>[3x]MIQGVIQKIAGPAVIAKGMLGARMYDICKVGEEGLVGEIIRLDGDTAFVQVYEDTSGLKVGEPVVSTGLPLAVELGPGMLNGIYDGIQRPLERIREKTGIYITRGVVVHALDREKKWAWTPMVKPGDEVRGGMVLGTVPEFGFTHKILVPPDVRGRVKEVKPAGEYTVEEPVVVLEDGTELKMYHTWPVRRARPVQRKLDPNTPFLTGMRILDVLFPVAMGGTAAIPGPFGSGKTVTQQSLAKWSNADVVVYVGCGERGNEMTDVLVEFPELTDPKTGGPLMHRTVLIANTSNMPVAAREASIYVGVTIAEYFRDQGFSVALMADSTSRWAEALREISSRLEEMPAEEGYPPYLAARLAAFYERAGKVITLGGEEGAVTIVGAVSPPGGDMSEPVTQSTLRIVGAFWRLDASLAFRRHFPAINWNGSYSLFTSALDPWYRENVAEDYPELRDAISELLQREAGLQEIVQLVGPDALQDAERLVIEVGRIIREDFLQQNAYHEVDAYCSMKKAYGIMKMILAFYKEAEAAIKRGVSIDEILQLPVLERIGRARYVSEEEFPAYFEEAMKEIQGAFKALA;>MDLLKKEYTGITYISGPLLFVENAKDLAYGAIVDIKDGTGRVRGGQVIEVSEEYAVIQVFEETTGLDLATTSVSLVEDVARLGVSKEMLGRRFNGIGKPIDGLPPITPEKRLPITGLPLNPVARRKPEQFIQTGISTIDVMNTLVRGQKLPIFSGSGLPANEIAAQIARQATVRPDLSGEGEKEEPFAVVFAAMGITQRELSYFIQEFERTGALSRSVLFLNKADDPTIERILTPRMALTVAEYLAFEHDYHVLVILTDMTNYCEALREIGAAREEIPGRRGYPGYMYTDLATIYERAGVVEGKKGSVTQIPILSMPDDDRTHPIPDLTGYITEGQIQLSRELHRKGIYPPIDPLPSLSRLMNNGVGKGKTREDHKQVSDQLYSAYANGVDIRKLVAIIGEDALTENDRRYLQFADAFERFFINQGQQNRSIEESLQIAWALLSMLPQGELKRISKDHIGKYYGQKLEEIWGAPQALD[3x];> MSQVSPTRMNLLQRRGQLRLAQKGVDLLKKKRDALVAEFFGLVREAMEARKALDQAAKEAYAALLLAQAFDGPEVVAGAALGVPPL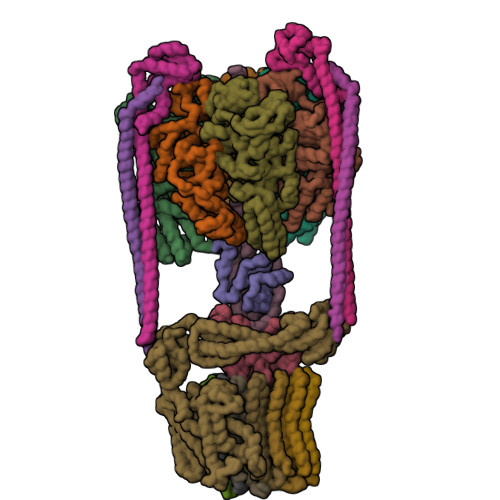EGVEAEVENVWGSKVPRLKATFPDGALLSPVGTPAYTLEASRAFRRYAEALIRVANTETRLKKIGEEIKKTTRRVNALEQVVIPGIRAQIRFIQQVLEQREREDTFRLKRIKGKIEAREAEEEGGRPNPQVEIGAGL;> MAVIADPETAQGFRLAGLEGYGASSAEEAQSLLETLVERGGYALVAVDEALLPDPERAVERLMRGRDLPVLLPIAGLKEAFQGHDVEGYMRELVRKTIGFDIKL;>MTGGLVLNAISRAGGAMGGLGLIKSLAEKEKQLLERLEAAKKEAEERVKRAEAEAKALLEEAEAKAKALEAQYRERERAETEALLARYRERAEAEAKAVREKAMARLDEAVALVLKEVLP[2x];>[2x]MSKLEAILSQEVEAEIQALLQEAEAKAEAVKREAEEKAKALLQARERALEAQYRAALRRAESAGELLVATARTQARGEVLEEVRRRVREALEALPQKPEWPEVVRKLALEALEALPGAKALVANPEDLPHLEAMARERGVELQAEPALRLGVRAVGAEGKTQVENSLLARMDRAWDAMSSKVAQALWG;> MADDFAYLNARVRVRRGTLLKESFFQEALDLSFADFLRLLSETVYGGELAGQGLPDVDRAVLRTQAKLVGDLPRLVTGEAREAVRLLLLRNDLHNLQALLRAKATGRPFEEVLLLPGTLREEVWRQAYEAQDPAGMAQVLAVPGHPLARALRAVLRETQDLARVEALLAKRFFEDVAKAAKGLDQPALRDYLALEVDAENLRTAFKLQGSGLAPDAFFLKGGRFVDRVRFARLMEGDYAVLDELSGTPFSGLSGVRDLKALERGLRCVLLKEAKKGVQDPLGVGLVLAYVKEREWEAVRLRLLARRAYFGLPRAQVEEEVVCP;> MIAPMEKLVLAGPKGRAKELLQSLQQAGVVHLETLRPEALSAYQLSPEERAELRRWEAVSAGAEHTLSLLGLEAEPARPFPEGLEAAEKALSPIQAHAEGLTRQKQELEEELALAQAYLEPLERLAALAHGLDKSPFLRVIPFLLTEKELPLVEEALRKALEDRYLLAHEAYAGGVAALVVVHRKEVDQAKAALSRAGVAELRLPGALGELPLSEAARRLKERAEAAPRELSEVRQHLAKLARESASTLQSLWTRAQDEVARLKALEELASGRFGFALLGYVPVKAKPKVEEALARHKESVVYAFEPVDEHHEADRIPVVLDNPPWAKPFELLVSFLNTPKYGTFDPTPVVPVFFPFWFGMIVGDIGYALLFYLVGRWLSGYVKRNEPLVIDLFALKLKPQVIGKLVHILNWMVFWTVVWGVIYGEFFGTFLEHLGVFGTPEHPGLIPILIHRIDTAKTANLLILLSVAFGVVLVFFGLALRAYLGLKHRHMAHFWEGVGYLGGLVGVLALAASYLGNLQAGWLQGLMYLGFGVFLLAVLMSRIWLMIPEIFTQAGHILSHIRIYAVGAAGGILAGLLTDVGFALAERLGLLGVLLGLLVAGVLHLLILLLTTLGHMLQPIRLLWVEFFTKFGFYEENGRPYRPFKSVREAQ;>MKKLLVTVLLAVFGALAFAAEEAAASGGLDRGLIAVGMGLAVGLAALGTGVAQARIGAAGVGAIAEDRSNFGTALIFLLLPETLVIFGLLIAFILNGRL[12x]> PSY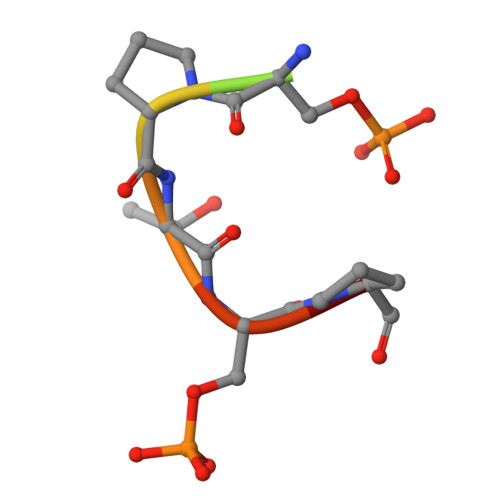SPTSPS TS is an essential enzyme for DNA replication. It catalyzes the transfer of a methylene group from the cofactor 5,10-methylenetetrahydrofolate (mTHF) to its substrate 2′-deoxyuridine-5′-monophosphate (dUMP) and produces thymidine-5′-monophosphate (dTMP) and dihydrofolate (DHF). KSHV encodes functional thymidylate synthase (kTS), which shares 70% sequence identity with hTS. The overall structure of kTS was found to have a similar structural conformation to hTS, except minor differences in ligand binding site and conformational variations in some amino acids.

The ternary kTS structure were determined by soaking apo kTS crystals with dUMP and raltitrexed since co-crystallization of kTS protein with ligands was unsuccessful. For the ternary kTS structure, an excellent density map of the ligands was observed except for the glutamate tail of raltitrexed. The ternary complex of kTS had an open conformation in which the catalytic Cys219 residue did not form a covalent bond with dUMP, which was also observed in rTS. In addition, the sulfhydryl group of ternary kTS was 3.3 Å away from the C6 atom of dUMP. The raltitrexed molecule was observed to bind to kTS at the active site by interactions with Phe104, Ile132, Asp242, Gly246, Phe249, Tyr282, and dUMP. There were less hydrophobic interactions with raltitrexed in kTS than in hTS. The Trp109 residue in hTS was found to interact with C7, C9, and CP1 of the raltitrexed molecule; the corresponding Trp133 residue in kTS did not interact with raltitrexed and was rotated about 60° away from raltitrexed. The distance between the Cα atoms of Tyr282 and Ile132 which were located at ligand binding site of kTS ternary complex was 18.8 Å, whereas the corresponding distance was 17.8 Å in hTS. C-terminal disorder might contribute to the open conformation in ternary kTS and rTS. Although the C-terminal region did not make crystal contacts with other symmetry-related molecules, we could not exclude the possibility that ternary kTS structure was not able to adopt a closed conformation due to the crystal lattice which may impede conformational changes to a closed conformation.

>[2x]PHEELQYLRQLREILCRGSDRLDRTGIGTLSLFGMQARYSLRDHFPLLTTKRVFWRGVVQELLWFLKGSTDSRELSRTGVKIWDKNGSREFLAGRGLAHRREGDLGPVYGFQWRHFGAAYVDADADYTGQGFDQLSYIVDLIKNNPHDRRIIMCAWNPADLSLMALPPCHLLCQFYVADGELSCQLYQRSGDMGLGVPFNIASYSLLTYMLAHVTGLRPGEFIHTLGDAHIYKTHIEPLRLQLTRTPRPFPRLEILRSVSSMEEFTPDDFRLVDYCPHPTIRM The final step in the pathway is catalyzed by a 2-epimerase, which utilizes UDP-2,3-diacetamido-2,3-dideoxy-d-glucuronic acid as its substrate. The focus of this investigation is on the ORF WP_011172736, which we demonstrate encodes for a 2-epimerase. We have also demonstrated that the T. thermophilus enzyme is allosterically regulated by UDP-GlcNAc. Whereas the sugar 2-epimerases that function on UDP-GlcNAc have been the focus of past biochemical and structural analyses, this is the first detailed investigation of a 2-epimerase that specifically utilizes UDP-2,3-diacetamido-2,3-dideoxy-d-glucuronic acid as its substrate.

The next structure solved in this investigation was that of the WT enzyme crystallized in the presence of its substrate, UDP-GlcNAc3NAcA at pH 5.0 (structures 2 and 3). The model was refined at 1.8 Å resolution with an overall R-factor of 18.2%. The α-carbons for the two subunits superimpose with an RMSD of 0.8 Å. As observed for other 2-epimerases, there is a significant closure of the gap between the N- and C-terminal domains upon UDP-sugar binding as highlighted in Figure 5. The uracil ring is positioned into the active site by the backbone amide and carbonyl oxygen of Val 265 and a water molecule. Glu 290 lies within hydrogen bonding distance to the ribosyl oxygens. The pyrophosphoryl moiety is surrounded by the side chains of Arg 12, His 208, and Ser 284. The pyranosyl moiety is anchored into the active site by the side chains of Gln 14, Lys 17, Asp 98, Glu 120, and Trp 307. In both subunits A and B, there is a chloride ion located within ∼3.2 Å of the side chain of Arg 12.

>[2x]MWVKILSVVGARPQFIKAAAVSRVLRASPGVREVLVHTGQHYDDNMSQVFFEELEIPDPDYHLGIGGGTHGQNTGRMLEAIEGVLLKEKPDWVLVYGDTDSTLAGALAAVKLHIPVAHVEAGLRSFNRRMPEEINRILTDHASDLLFAPTETAVQNLLREGIPENRIHLVGDVMYDAALHYGAKAERKSRILERLGLQAKGYVLATIHRAENTDDQERLRVILEALAEVHQEVPVVFPVHPRTRKRAEAFGLGSYLEKVVALEPVGYLDMVMLEKNARLIVTDSGGVQKEAYFYRVPCVTVREETEWVELLKAEWNYLAAPQNAKDLALTILHRMRTKGVEIDLYGDGRASQKISDFLRKVGIRTLEHHHHHH>[10x]MGSSHHHHHHSQDPEQSTPDEVNAALDRLLIADALAQLSAEHRAVIQRSYYR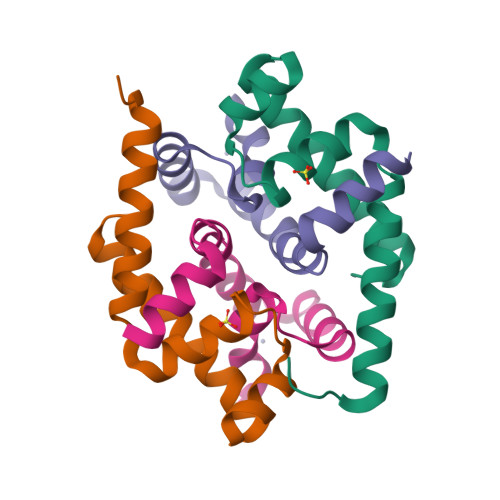GWSTAQIATDLGIAEGTVKSRLHYAVRALRLTLQELGVTR;>MTMPLRGLGPPDDTGVREVSTGDDHHYAMWDAAYVLGALSAADRREFEAHLAGCPECRGAVTELCGVPALLSQLDRDEVAAISESAPTVVASGLSPELLPSLLAAVHR[10x]> MMRRAYPEGPPPSYESVMQQAMAAAAAMQPPLEAPYVPPRYLAPTEGRNSIRYSELAPLYDTTRLYLVDNKSADIASLNYQNDHSNFLTTVVQNNDFTPTEASTQTINFDERSRWGGQLKTIMHTNMPNVNEFMYSNKFKARVMVSRKTPNGVTVTDGSQDILEYEWVEFELPEGNFSVTMTIDLMNNAIIDNYLAVGRQNGVLESDIGVKFDTRNFRLGWDPVTELVMPGVYTNEAFHPDIVLLPGCGVDFTESRLSNLLGIRKRQPFQEGFQIMYEDLEGGNIPALLDVDAYEKSKEESAAAATAAVATASTEVRGDNFASPAAVAAAEAAETESKIVIQPVEKDSKDRSYNVLPDKINTAYRSWYLAYNYGDPEKGVRSWTLLTTSDVTCGVEQVY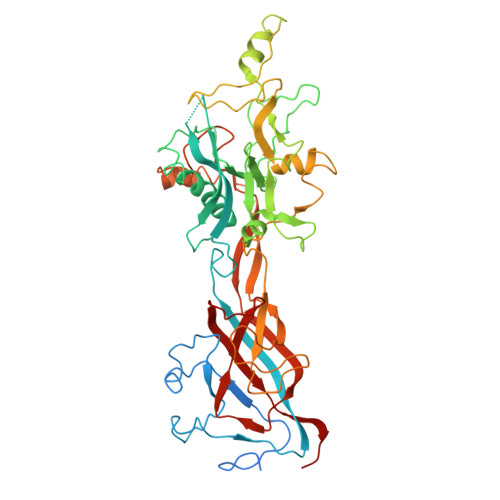WSLPDMMQDPVTFRSTRQVSNYPVVGAELLPVYSKSFFNEQAVYSQQLRAFTSLTHVFNRFPENQILVRPPAPTITTVSENVPALTDHGTLPLRSSIRGVQRVTVTDARRRTCPYVYKALGIVAPRVLSSRTF>[3x]MRGSFVEMVDNLRGKSGQGYYVEMTVGSPPQTLNILVDTGSSNFAVGAAPHPFLHRYYQRQLSSTYRDLRKGVYVPYTQGKWEGELGTDLVSIPHGPNVTVRANIAAITESDKFFINGSNWEGILGLAYAEIARPDDSLEPFFDSLVKQTHVPNLFSLQLCGAGFPLNQSEVLASVGGSMIIGGIDHSLYTGSLWYTPIRREWYYEVIIVRVEINGQDLKMDCKEYNYDKSIV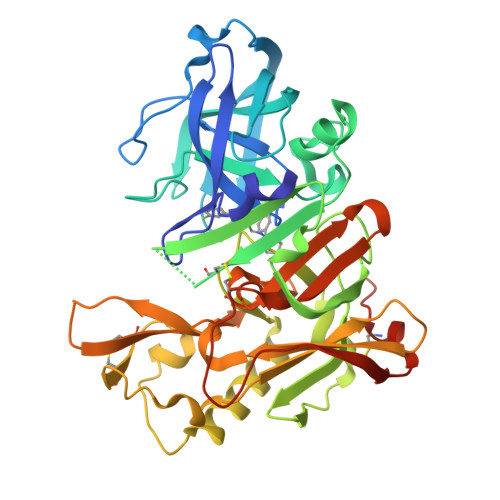DSGTTNLRLPKKVFEAAVKSIKAASSTEKFPDGFWLGEQLVCWQAGTTPWNIFPVISLYLMGEVTNQSFRITILPQQYLRPVEDVATSQDDCYKFAISQSSTGTVMGAVIMEGFYVVFDRARKRIGFAVSACHVHDEFRTAAVEGPFVTLDMEDCGYNIPQTDESRSHHHHHH>[2x]REARGATEEPSPPSRALYFSGRGEQLRLRADLELPRDAFTLQVWLRAEGGQRSPAVITGLYDKCSYISRDRGWVVGIHTISDQDNKDPRYFFSLKTDRARQVTTINAHRSYLPGQWVYLAATYDGQFMKLYVNGAQVATSGEQVGGIFSPLTQKCKVLMLGGSALNHNYRGYIEHFSLWKVARTQREILSDMETHGAHTALPQLLLQENWDNVKHAWSPMKDGSSPKVEFSNAHGFLL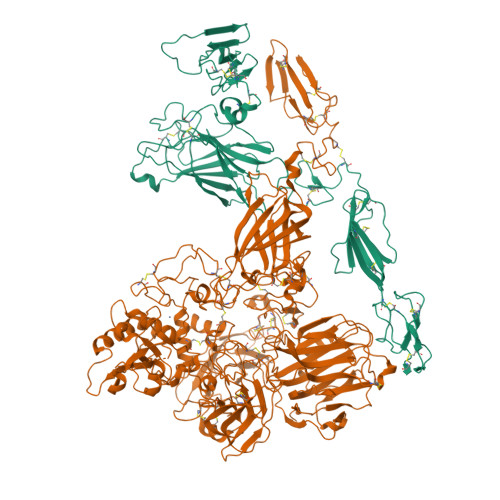DTSLEPPLCGQTLCDNTEVIASYNQLSSFRQPKVVRYRVVNLYEDDHKNPTVTREQVDFQHHQLAEAFKQYNISWELDVLEVSNSSLRRRLILANCDISKIGDENCDPECNHTLTGHDGGDCRHLRHPAFVKKQHNGVCDMDCNYERFNFDGGECCDPEITNVTQTCFDPDSPHRAYLDVNELKNILKLDGSTHLNIFFAKSSEEELAGVATWPWDKEALMHLGGIVLNPSFYGMPGHTHTMIHAIGHSLGLYHVFRGISEIQSCSDPCMETEPSFETGDLCNDTNPAPKHKSCGDPGPGNDTCGFHSFFNTPYNNFMSYADDDCTDSFTPNQVARMHCYLDLVYQGWQPSRKPAPVALAPQVLGHTTDSVTLEWFPPIDGHFFERELGSACHLCLEGRILVQYASNASSPMPCSPSGHWSPREAEGHPDVEQPCKSSVRTWSPNSAVNPHTVPPACPEPQGCYLELEFLYPLVPESLTIWVTFVSTDWDSSGAVNDIKLLAVSGKNISLGPQNVFCDVPLTIRLWDVGEEVYGIQIYTLDEHLEIDAAMLTSTADTPLCLQCKPLKYKVVRDPPLQMDVASILHLNRKFVDMDLNLGSVYQYWVITISGTEESEPSPAVTYIHGSGYCGDGIIQKDQGEQCDDMNKINGDGCSLFCRQEVSFNCIDEPSRCYFHDGDGVCEEFEQKTSIKDCGVYTPQGFLDQWASNASVSHQDQQCPGWVIIGQPAASQVCRTKVIDLSEGISQHAWYPCTISYPYSQLAQTTFWLRAYFSQPMVAAAVIVHLVTDGTYYGDQKQETISVQLLDTKDQSHDLGLHVLSCRNNPLIIPVVHDLSQPFYHSQAVRVSFSSPLVAISGVALRSFDNFDPVTLSSCQRGETYSPAEQSCVHFACEKTDCPELAVENAYLNCSSSDRYHGAQCTVSCRTGYVLQIRRDDELIKSQTGPSVTVTCTEGKWNKQVACEPVDCSIPDHHQVYAASFSCPEGTTFGSQCSFQCRHPAQLKGNNSLLTCMEDGLWSFPEALCELMCLAPPPVPNADLQTARCRENKHKVGSFCKYKCKPGYHVPGSSRKSKKRAFKTQCTQDGSWQEGACVPVTCDPPPPKFHGLYQCTNGFQFNSECRIKCEDSDASQGLGSNVIHCRKDGTWNGSFHVCQEMQGQCSVPNELNSNLKLQCPDGYAIGSECATSCLDHNSESIILPMNVTVRDIPHWLNPTRVERVVCTAGLKWYPHPALIHCVKGCEPFMGDNYCDAINNRAFCNYDGGDCCTSTVKTKKVTPFPMSCDLQGDCACRDPQAQEHSRKDLRGYSHGSGPTRTRPLEQKLISEEDLAANDILDYKDDDDKV N-[(1R)-1-(4-methoxyphenyl)-2-oxo-2-{[4-(trimethylsilyl)phenyl]amino}ethyl]-N-methyl-3-oxo-2,3-dihydro-1,2-oxazole-5-carboxamide | C23 H27 N3 O5 Si | 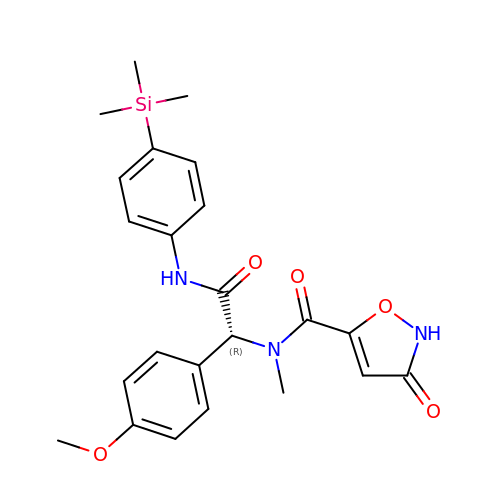RQLIWGALGGOPGM-OAQYLSRUSA-N> MPITIGNGFLKSEILTNSPRNTKEAW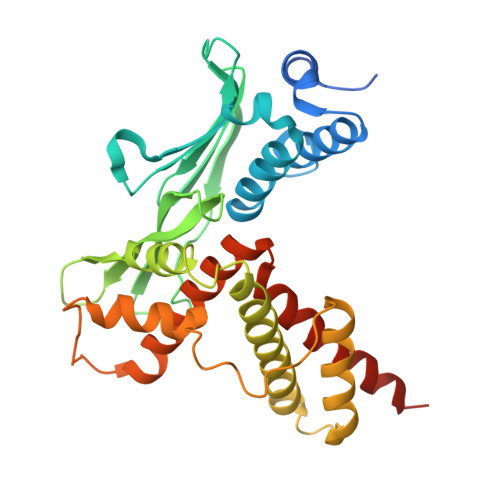WKVLWEKIKDFFFSTGKAKADRCLHEMLFAERAPTRERLTEIFFELKELACASQRDRFQVHNPHENDATIILRIMDQNEENELLRITQNTDTFSCEVMGNLYFLMKDRPDILKSHPQMTAMIKRRYSEIVDYPLPSTLCLNPAGAPILSVPLDNIEGYLYTELRKGHLDGWKAQEKATYLAAKIQSGIEKTTRILHHANISESTQQNAFLETMAMCGLKQLEIPPPHTHIPIEKMVKEVLLADKTFQAFLVTDPSTSQSMLAEIVEAISDQVFHAIFRIDPQAIQKMAEEQLTTLHVRSEQQSGCLCCFL;> TKEGMLHYKAGTSYLGKEHWKTCFVVLSNGILYQYPDRTDVIPLLSVNMGGEQCGGCRRANTTDRPHAFQVILSDRPCLELSAESEAEMAEWMQHLCQAVSKGVIPQGVAPS> MSSDPFKKVERDYHNERSVHKHFASYPLKFWWGLNKF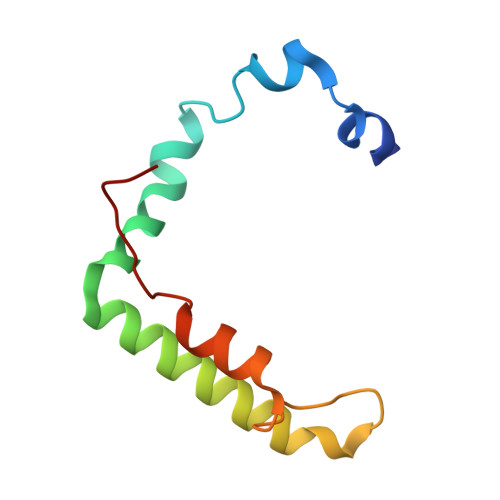ETIQGIHSILGNAADLVVSTLSFIPGVQGRNNASYIENSIRVTRFRGFDDKTQ>[8x]GNVTQAF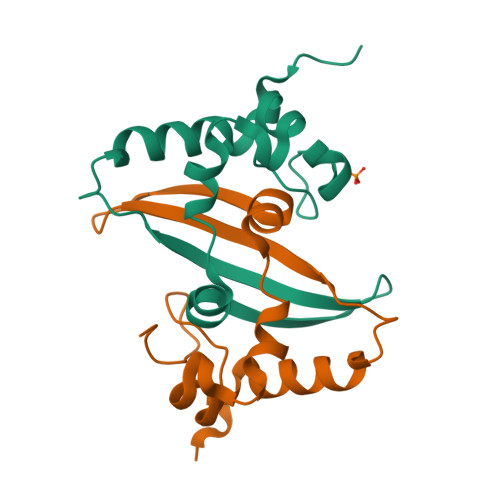GRRGPEQTQGNFGDQELIRQGTDYKHWPQIAQFAPSASAFFGMSRIGMEVTPSGTWLTYTGAIKLDDKDPNFKDQVILLNKHIDAYKTFPPTE N-methyl-4-propanoyl-1H-pyrrole-2-carboxamide | C9 H12 N2 O2 | 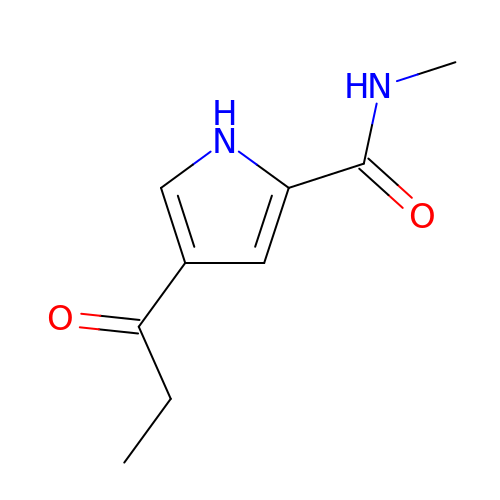CWMKCPQGJKUMBN-UHFFFAOYSA-N> GSHMEPLKVEKFATANRGNGLRAVTPLRPGELLFRSDPLAYTVCKGSRGVVCDRCLLGKEKLMRCSQCRVAKYCSAKCQKKAWPDHKRECKCLKSCKPRYPPDSVRLLGRVVFKLMDGAPSESEKLYSFYDLESNINKLTEDRKEGLRQLVMTFQHFMREEIQDASQLPPAFDLFEAFAKVICNSFTICNAEMQEVGVGLYPSISLLNHSCDPNCSIVFNGPHLLLRAVRDIEVGEELTICYLDMLMTSEERRKQLRDQYCFECDCFRCQTQDKDADMLTGDEQVWKEVQESLKKIEELKAHWKWEQVLAMCQAIISSNSERLPDINIYQLKVLDCAMDACINLGLLEEALFYGTRTMEPYRIFFPGSHPVRGVQVMKVGKLQLHQGMFPQAMKNLRLAFDIMRVTHGREHSLIEDLILLLEECDANIRAS

The drug target in this study is the epigenetic regulator SET (suppressor of variegation, enhancer of zeste, trithorax) and MYND (myeloid-Nervy-DEAF1) domain-containing protein 3 (SMYD3). This belongs to the SMYD family which consists of five proteins (SMYD1 to SMYD5) that have similar structures and domain compositions. The SMYD family plays an intrinsic role in both normal and diseased states, with overexpression of SMYD2 found in cancerous tumours specifically oesophageal, bladder, and stomach whilst SMYD3 overexpression is detected in liver, colon, and breast carcinomas.

Screening was done in parallel against SMYD3 alone or SMYD3 with the active site blocked by a tight binding inhibitor. In total, 20 fragments were selected as hits, of which half apparently targeted the active site and half targeted other sites. Twelve of the hits were selected for structural analysis using X-ray crystallography in order to identify binding sites and modes of binding. Four of the hits were successfully identified in crystal structures with SMYD3; the others did not show any electron densities for ligands in the crystals. The hits identified using this novel screening approach were confirmed via X-ray crystallography and revealed that SMYD3 has multiple ligand binding sites, distinct from the active site that can be targeted with fragments. Moreover, the electron densities of the crystallisable hits were weak. Fragment FL01507 is considered the least reliable starting point for generation of new ligands, since the associated electron density was not as clear and the binding site had not been predicted. However, further work is clearly required to evolve the fragments into ligands amenable to a structure-based approach and to explore their interactions with the newly identified binding sites.>[60x]MGSSHHHHHHSSSAALEVLFQGPMELFNRVGRVLKSQLTHWQ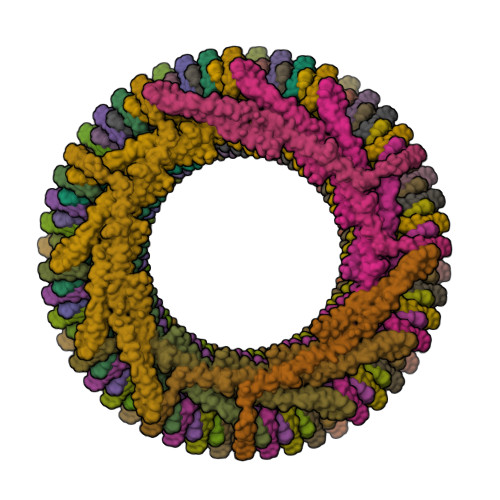QQQEAPEDLLERLLGEMELELIELRRALAQTIATFKSTERQRDAQQLIAQRWYEKAQAALDRGNEQLAREALGQRQSYQSHTEALGKSLGEQRALVEQVRGQLQKLERKYLELKSQKNLYLARLKSAIAAQKIEEIAGNLDNASASSLFERIETKILELEAERELLNPPPSPLDKKFEQWEEQQAVEATLAAMKARRSLPPPSS Drosophila off-track or OTK is a transmembrane protein that plays important roles in development and reproduction. Sequence analysis suggests that OTK is a single-pass transmembrane protein with five extracellular immunoglobulin (Ig)-like domains, which show homology with neural cell adhesion molecules (Pulido et al., 1992). The intracellular domain shows homology with receptor tyrosine kinases; however, the kinase domain is probably not active since conserved residues implicated in autophosphorylation are altered in OTK. Functionally, OTK has been reported to bind Drosophila Plexin A (PlexA), a receptor for the axon guidance molecule semaphorin 1a (Sema1a).

We crystallized the OTK ectodomain and determined the crystal structure of the last three D3-D5 domains (OTK3-5) to 1.97 Å resolution. The overall architecture of OTK3-5 is arranged in an extended conformation with substantial curvature resembling a boomerang shape. OTK D3-D5 domains adopt the I-set fold of the Ig-like domain superfamily which has been found in many cell adhesion molecules, protein tyrosine kinase receptors, and signaling molecules. The asymmetric unit contains two chains, and structural superposition of these chains revealed that D3 and D5 can re-orientate relative to the D4 domain by 28° and 40° about hinge points located in the D3-D4 and D4-D5 linkers, respectively, giving clear evidence for interdomain flexibility. The interdomain flexibility is presumably allowed by the small interdomain interfaces and a lack of strong interactions between the individual domains. Sequence analysis of potential protease cleavage sites revealed an internal furin site RGKR at positions 235–238, located between D2 and D3, suggesting that the ectodomain of OTK1-5 was cleaved by furin protease during crystallization. N-linked glycans were clearly visible and unambiguously fitted into the electron density at Asn336, 417, 429, 444, 457, and 524. A close inspection of the electrostatic potential on the OTK3-5 surface revealed two substantial regions of basic charge on D3 and D4. In the crystal structure, both basic patches interact with well-ordered sulfate ions from the crystallization solution. Binding of sulfate ions and notable similarity to consensus sequences (Hileman et al., 1998) for heparin binding suggest that both patches represent potential glycosaminoglycan (GAG) binding sites.

>[2x]ETGSSRFQRVPQSQSVVENESVKFECESTDSYSELHYDWLHNGHRIAYDKRVHQIGSNLHIEAVRRTEDVGNYVCIATNLASGAREASPPAKLSVIYLESASVQLLGSNRNELLLKCHVEGASGDLEPLEIEWYRNSEKLSTWKNVQLDQHRLIIRQPGSEDDGLYRCTASNAAGRVMSKQGYVYQSSVKCLPRLPRRKNEKMMESWDKQTFLCRGKRGGAAGLEALPAAPEDLRIVQGPIGQSIIKEGEPTALTCLYELPDELKNQRIQLRWRKDGKLLRQVELGGSAPIPGHSFDSGKDALLREDARLVLHKQNGTLSFASIIASDAGQYQCQLQLEAHAPINSSPGILEVIEQLKFVPQPTSKNLELDAVVAKVHCKAQGTPTPQVQWVRDGENTTLPDHVEVDANGTLIFRNVNSEHRGNYTCLATNSQGQINATVAINVVVTPKFSVPPVGPIETSEQGTVVMHCQAIGDPKPTIQWDKDLKYLSENNTDRERFRFLENGTLEIRNVQVEDEGSYGCTIGNSAGLKREDVQLVVKTTGDGFAPEESGGDGFLVTRGTKHHHHHH> MA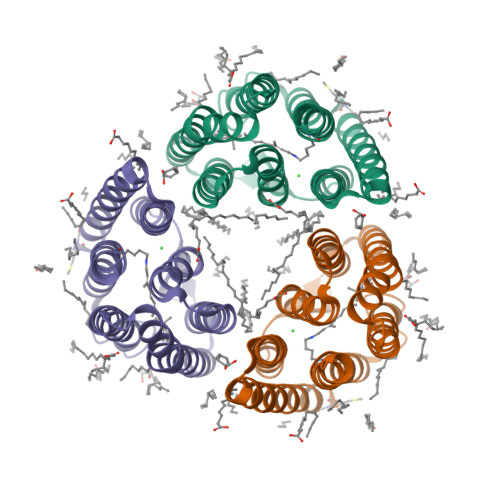QIWLWIGVIGMALGSIFFGIGAHNAKNERWKILFTINFFICAIATGLYLSMALGQGRSVIAGRPTVWVRYITWFLSTPLLILDLTFLGKTSLPITASLLGANAYMIATGFVATISADRTIGHIWYVVSCFAFLATVYLLVNQYRKQAERNYPQAKKVFRKLLSVHLVLWTLYPIVWLLGNTGFNAVNQGTETMFYTILDITSKVGFGFLSLNSMHTLEKNTESVSSYESSTI>[2x]GSHMRSRRVDVMDVMNRLILAMDLMNRDDALRVTGEVREYIDTVKIGYPLVLSEGMDIIAEFRKRFGCRIIADFKVANIPETNEKICRATFKAGADAIIVHGFPGADSVRACLNVAEEMGREVFLLTEMSHPGAEMFIQGAADEIARMGVDLGVKNYVGPSTRPERLSRLREIIGQDSFLISPGVGAQGGDPGE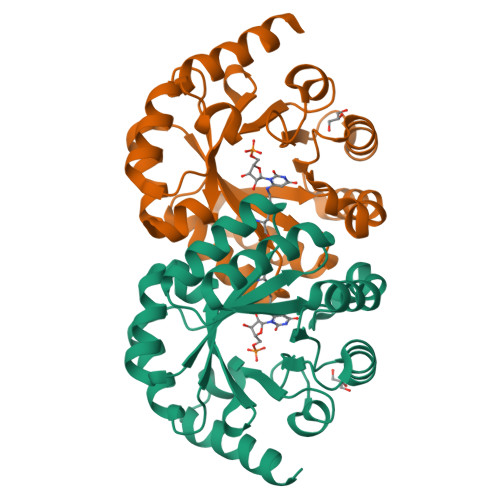TLRFADAIIVGRSIYLADNPAAAAAGIIESIKDLRIPEDPAANKARKEAELAAATAEQ>[2x]MGHHHHHHHAMEN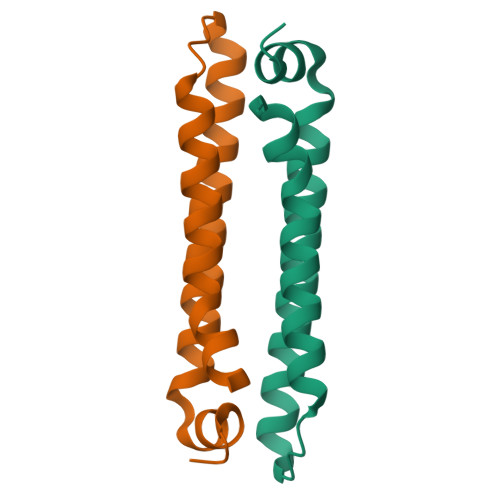LYFQGHMTNMSCAYELIKSLPAKLEQLAQETQATIQTLMIADPNVNKDLRAFCEFLTVQHQRAYRATNSLLIKPRVAAALRGEE> MGGGGTDRVRRSEAITHGTPFQKAAALVDLAEDGIGLPVEILDQSSFGESARYYFIFTRLDLIWSLNYFALLFLNFFEQPLWCEKNPKPSCKDRDYYYLGELPYLTNAESIIYEVITLAILLVHTFFPISYEGSRIFWTSRLNLVKVACVVILFVDVLVDFLYLSPLAFDFLPFRIAPYVRVIIFILSIRELRDTLVLLSGMLGTYLNILALWMLFLLFASWIAFVMFEDTQQGLTVFTSYGATLYQMFILFTTSNNPDVWIPAYKSSRWSSVFFVLYVLIGVYFVTNLILAVVYDSFKEQLAKQVSGMDQMKRRMLEKAFGLIDSDKNGEIDKNQCIKLFE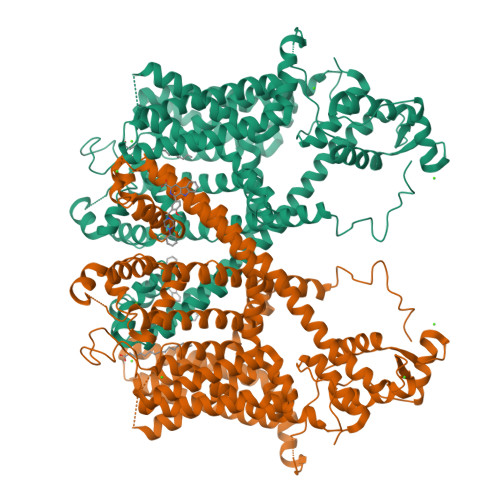QLTNYRTLPKISKEEFGLIFDELDDTRDFKINKDEFADLCQAIALRFQKEEVPSLFEHFPQIYHSALSQQLRAFVRSPNFGYAISFILIINFIAVVVETTLDIEESSAQKPWQVAEFVFGWIYVLEMALKIYTYGFENYWREGANRFDFLVTWVIVIGETATFITPDENTFFSNGEWIRYLLLARMLRLIRLLMNVQRYRAFIATFITLIPSLMPYLGTIFCVLCIYCSIGVQVFGGLVNAGNKKLFETELAEDDYLLFNFNDYPNGMVTLFNLLVMGNWQVWMESYKDLTGTWWSITYFVSFYVITILLLLNLVVAFVLEAFFTELDLEEEEKCQGQDSQEKRNRRRSAGSKSRSQRVDTLLHHMLGDELSKPECSTSDT(4R)-2-[(1,3-benzoxazol-2-yl)amino]-4-(4-chloro-1H-pyrazol-5-yl)-4,6,7,8-tetrahydroquinazolin-5(1H)-one | C18 H15 Cl 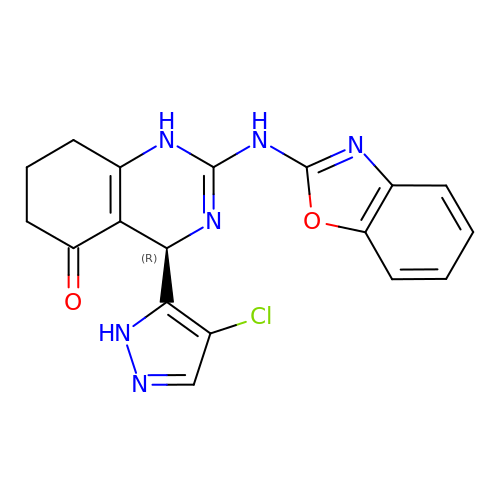N6 O2 | ORBGGGFENULXFO-MRXNPFEDSA-N>[2x]MEAVKTFNSELYSLMDMKPPISKAKMTQITKAAIKAIKFYKHVVQSVEKFIQKCKPEYKVPGLYVIDSIVRQSRHQFGQEKDVFAPRFSNNIISTFQNLYRC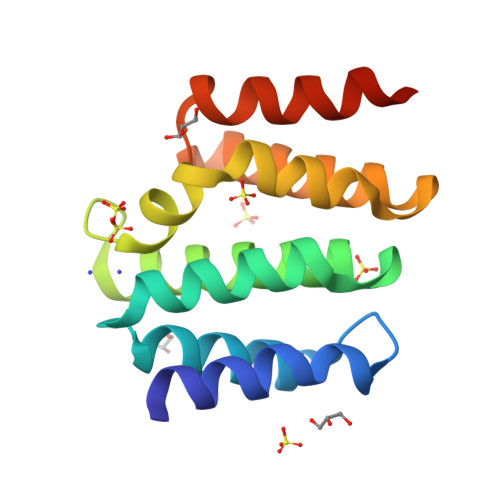PGDDKSKIVRVLNLWQKNNVFKSEIIQPLLDMAAALEHHHHHH> QEAQTELPQARISCPEGTNAYRSYCYYFNEDRETWVDADLYCQNMNSGNLVSVLTQAEGAFVASLIKESGTDDFNVWIGLHDPKKNR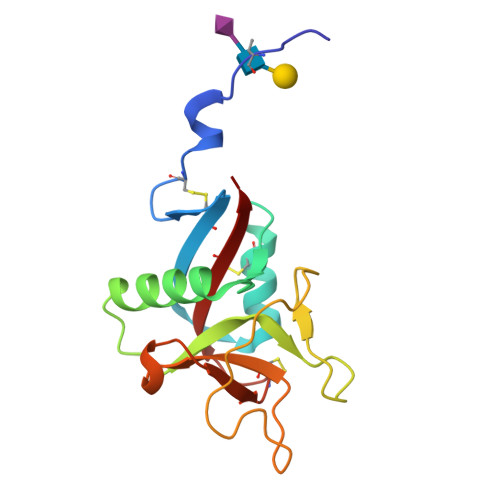AWHWSSGSLVSYKSWGIGAPSSVNPGYCVSLTSSTGFQKWKDVPCEDKFSFVCKFKN> MSIVTKSIVNADAEARYLSPGELDRIKAFVTGGAARLRIAETLTGSRET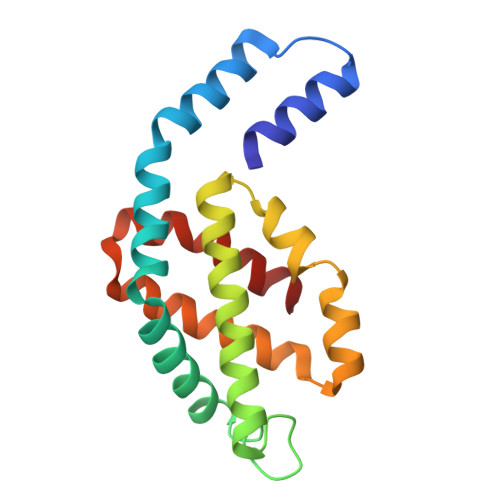IVKQAGDRLFQKRPDIVSPGGNAYGEEMTATCLRDMDYYLRLVTYGVVSGDVTPIEEIGLVGVREMYRSLGTPIEAVAQSVREMKEVASGLMSSDDAAEASAYFDFVIGKMS>MTNKVLTISSYVCSGFVGNRCGMIILDSFQIQSIFVLTTHLANHTGYPVVGGSGVLLNDFISIMDSLEVNHLDKDIEFLVTGYFPSSDLVYETINRVKRIKDNKKVYFLCDPILGDNGKMYTKSEVQDSMKEL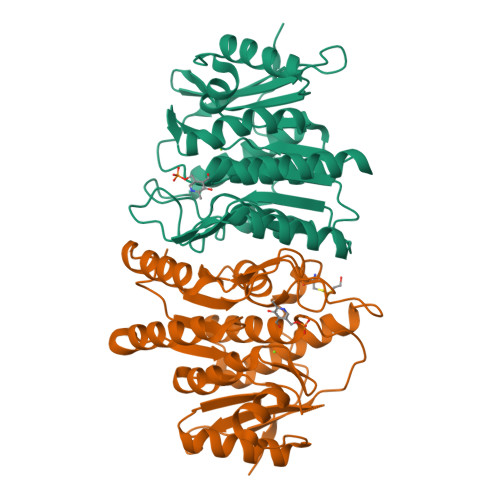IKYADIITPNATELSFLTGLEVNSVSEAIKACHILHEQGIPVILVTSIKEGNDIILLCSFKDTLNNKNFTIKIPRIEGDFTGVGDTLTYILLSWIIKGIPLEHAVNRAISTLQTILRNTVGTAEINIINCIPYLKGTEESFTITYILEHHHHHH[2x]>GMTQPHQIILLAHGSSDARWCETFEKLAEPTVESIENAAIAYMELAEPSLDTIVNRAKGQGVEQFTVVPLFLAAGRHLRKDVPAMIERLEAEHGVTIRL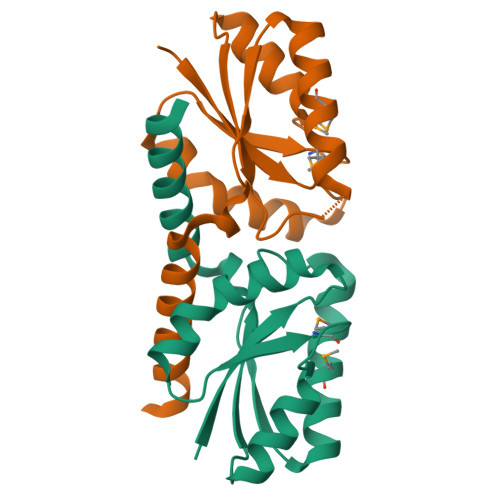AEPIGKNPRLGLAIRDVVKEELERSEH[2x]> MAEITETQESLPPFRMGEVGSLGLKVKNGRIYEEPRQALRFPESIKTFQLMMRDPAVAASVNIIKMFVRKVNWRFVPPKGKEQDPKMLERADFFNSLMDDMEHDWADFINSVMSFCTYGFCVNEKVYKKRQGKKGKYQSKFDDG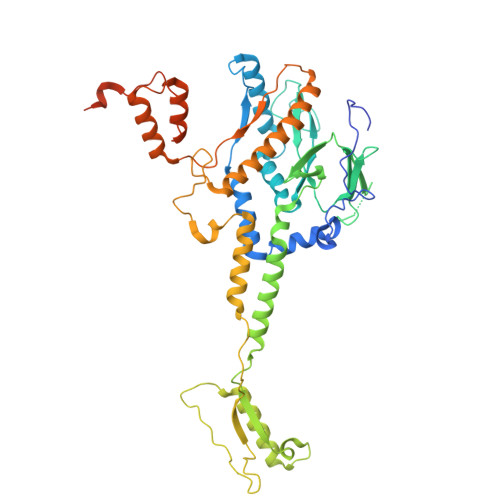LIGWAKLPIRNQSTLDKWYFDEDFRKVTGVRQNLRNVSHIAGAINLGERPLTRKLPRAKFMLFKYDDEYGNPEGRSPLLNAYVPWKYKVQIEEYEAVGVSRDLVGMPKIGLPPDYLDENAEPEKKAFVQYCKTVVNDMIANDRAGLIWPRYIDPDTKEDIFEFSLVSRQGAKAYDTGSIIDRYSKQIMMAFMSDVLAMGQSKYGSFSLADSKTSLLAMSVDILLKQIKNVINRDLVAQTYALNMWDDEEHVQITYDDIETPDLEAIGSYIQKTVAVGALEVDKELSNKLREHIGLPPADESQPVSEKLSPNSQSRSGDGYKTAGEGTAKTPSAKDPSTANKANK>[2x]XE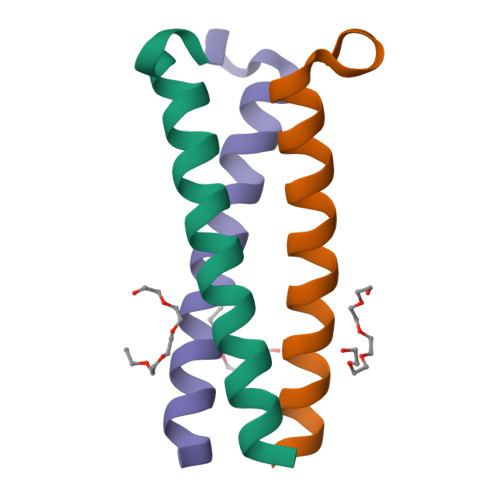VEALEKKVAALELKVQKLEKKVEALEHGWDGR1-[(3~{R})-3-[4-azanyl-3-[1-[2,2-bis(fluoranyl)-2-phenyl-ethyl]-1,2,3-triazol-4-yl]pyrazolo[3,4-d]pyrimidin-1-yl]piperidin-1-yl]propan-1-one 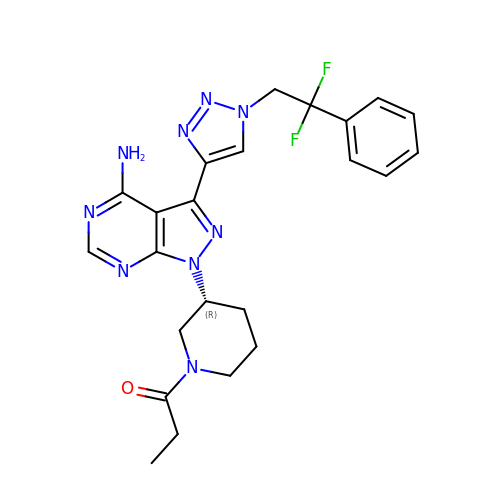| C23 H25 F2 N9 O | RKZKJXWXRLEVRP-MRXNPFEDSA-N> MNIGLLEALDQLEEEKGISKEEVIPILEKALVSAYR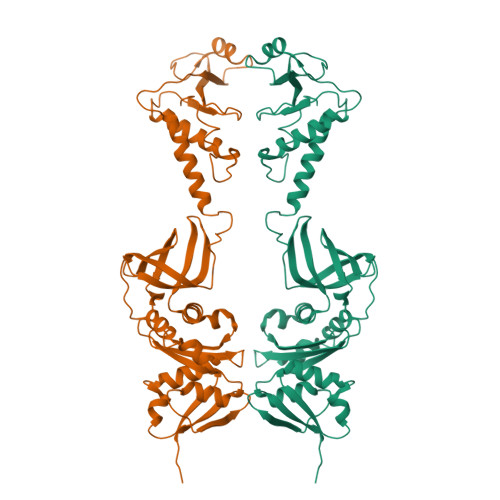KNFGNSKNVEVVIDRNTGNIKVYQLLEVVEEVEDPATQISLEEAKKIDPLAEVGSIVKKELNVKNFGRIAAQTAKQVLIQRIRELEKEKQFEKYSELKGTVTTAEVIRVMGEWADIRIGKLETRLPKKEWIPGEEIKAGDLVKVYIIDVVKTTKGPKILVSRRVPEFVIGLMKLEIPEVENGIVEIKAIAREPGVRTKVAVASNDPNVDPIGACIGEGGSRIAAILKELKGEKLDVLKWSDDPKQLIANALAPATVIEVEILDKENKAARVLVPPTQLSLAIGKGGQNARLAAKLTGWKIDIKPIMNL>SMELNSQFNAFLTNIRPTDPQKEDWKGGAKTLRERLNNYEPLKDIVVSTFLQGSIRRSTAIRPLNGKRPDVDIVVVTNLDHNQIAPQEAMDLFVPFLEKYYPEKWVPQGRSFGITLSYVELDLVITAIPASGEEKNLLEQLYRSESVLTVNSLEEQKDWRLNKSWKPSESGLFISNSANIQDAPLSEWKAHPLVLPDRDENKWGRTHPLAQIRWTAEKNRACNGHYINLVRAVKWWRQQNSDNLPKYPKGYPLEHLIGNALDDGTPSMGKGLVQLIDTFLSRWAYVYSLRSKPSLPDHGVE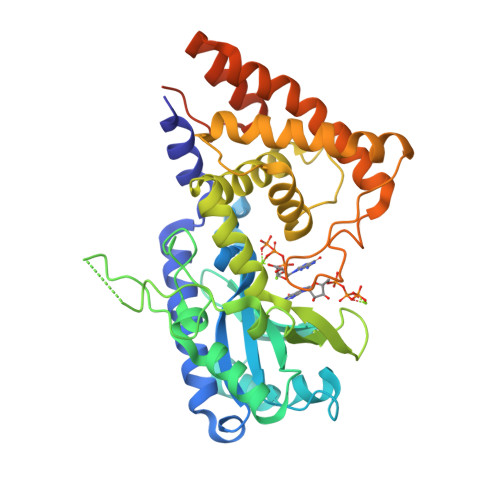EHDVLARLSAEDFCLFYEGLEDAAIIARSALASQDPKESAELWRKLFGTKFPFPGPQGGDRSSGFTAPTQPAEPQKTGRFA[2x]>DYKDDDDKAEVKKIPTMIEGFDDISHGGLPQGATTLVSGTSGTGKTLFAVQFLYNGITIFNEPGIFVTFEESPQDIIKNALSFGWNLQSLIDQGKLFILDASPDPDGQEVAGDFDLSALIERIQYAIRKYKATRVSIDSVTAVFQQYDAASVVRREIFRLAFRLAQLGVTTIMTTERVDEYGPVARFGVEEFVSDNVVILRNVL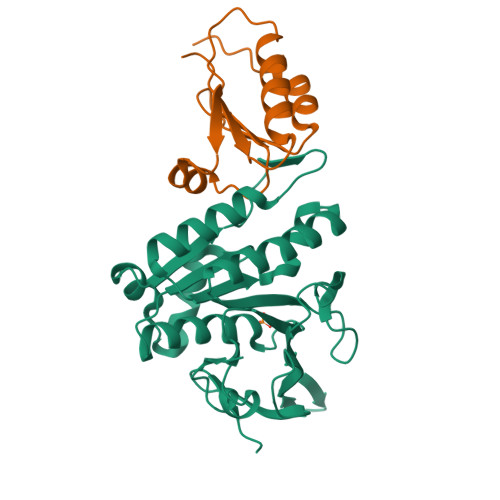EGERRRRTVEILKLRGTTHMKGEYPFTINNGINIFDYKDDDDK[6x];>DYKDDDDKALSLLLFVANRPGDEEETAAIQAHIQQLPSNFSFELKVVPIGEQPYLLEEYKLVATPALIKVRPEPRQTLAGRKLLQKVDYWWPRWQREVALDYKDDDDK[6x]>MATKLDYEDAVFYFVDDDKICSRDSIIDLIDEYITWRNHVIVFNKDITSCGRLYKELMKFDDVAIRYYGIDKINEIVEAMSEGDHYINFTKVHDQESLFATIGICAKITEHWGYKKISESRFQSLGNITDLMTDDNINILILFL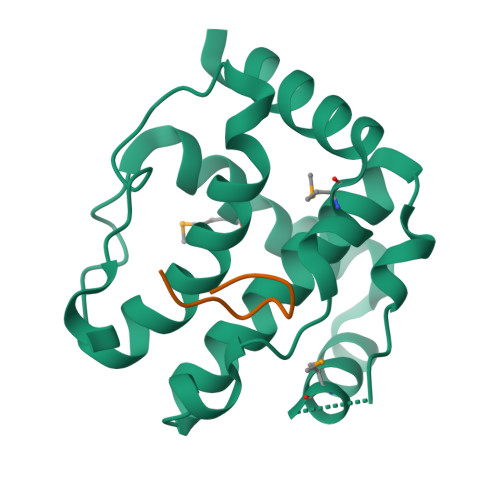EKKLN[2x];>[3x]SFGSRSDSRGKSSFFSDRGS> RVLQVDIVPSQGEISVGESKFFLCQVAGDAKDKDI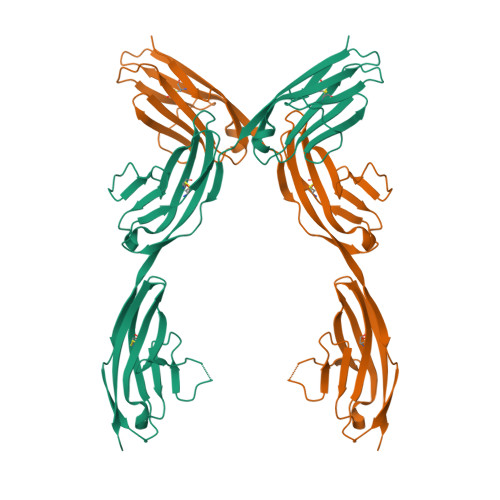SWFSPNGEKLSPNQQRISVVWNDDDSSTLTIYNANIDDAGIYKCVVTAEDGTQSEATVNVKIFQKLMFKNAPTPQEFKEGEDAVIVCDVVSSLPPTIIWKHKGRDVILKKDVRFIVLSNNYLQIRGIKKTDEGTYRCEGRILARGEINFKDIQVIVNVPPTVQARQSIVNATANLGQSVTLVCDADGFPEPTMSWTKDGEPIENEEEDDEKHIFSDDSSELTIRNVDKNDEAEYVCIAENKAGEQDASIHLKVFAK> CGCGAA;> TT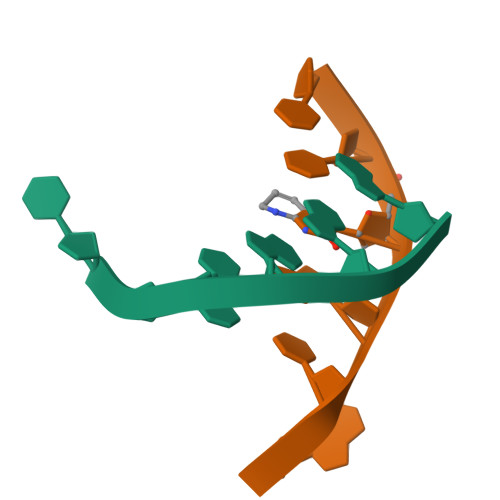XGCG>HHHHHHFNLPPGNYKKPKLLYCSNGGHFLRILPDGTVDGTRDRSDQHIQFQLSAESVGEVYIKSTETGQYLAMDTDGLVYGSQTPNEECLFLERLEENHYNTYISKKHAEKNWFLGIKKNGSVKRGPRTHYGQKA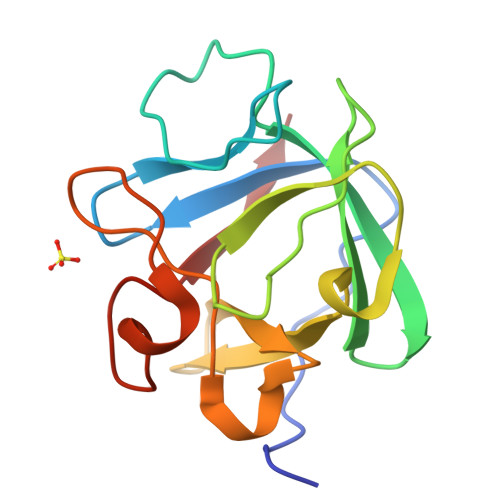ILFLPLPV[4x]>[4x]MGATDRTPPSNAILSNSNSDNNSTQGSQSGTVTKTPNPEATGSLSGKPTQIPPLSDEVTTRSLIRENQSAVTLANKGYDVVQNPEVLGPKNPDYTINGQVFDNYAPATGNVRNIATTISNKVSSGQASNIVVNLADSSASPAAIEAQINSYPIPGLGKVIVIDKLGNITIIKPKGN;>MAIDLFCYLSIDRGAAESDLNKIRSNHSELFEGKFLISPVRDADFSLKEIAAEHGLVAESFFL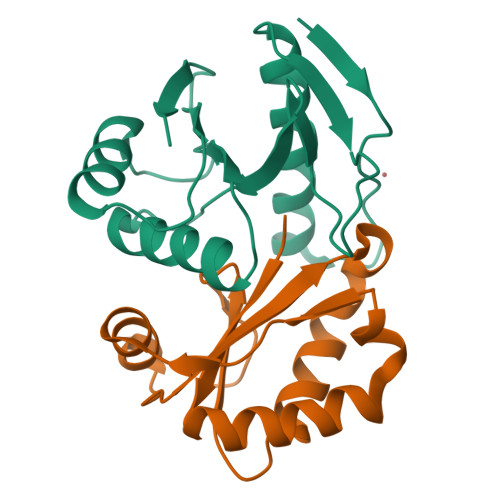VSLNDKNSADLIPIVSKILVDGFNGGAILILQDNEYRRTSLEHHHHHH[4x]>SSHVETRAHAEERLLKKLFSGYNKWSRPVANISDVVLVRFGLSIAQLIDVDEKNQMMTTNVWVKQEWHDYKLRWDPADYENVTSIRIPSELIWRPDIVLYNNADGDFAVTHLTKAHLFHDGRVQWTPPAIYKSSCSIDVTFFPFDQQNCTMKFGSWTYDKAKIDLVNMHSRVDQLDFWESGEWVIVDAVGTYNTRKYECCAEIYPDITYAFVIRRLPLFYTINLIIPCLLISCLTVLVFYLPSECGEKITLCISVLLSLTVFLLLITEIIPSTSLVIPLIGEYLLFTMIFVTLSIVITVFVLNVHHRSPRTHTMPTWVRRVFLDIVPRLLLMKRPSVVDTDFERSVKEDWKYVAMVIDRIFLWMFIIVCLLGTVGLFLPPWLAGMI[2x];>[3x]TDTEERLVEHLLDPSRYNKLIRPATNGSELVTVQLMVSLAQLISVHEREQIMTTNVWLTQEWEDYR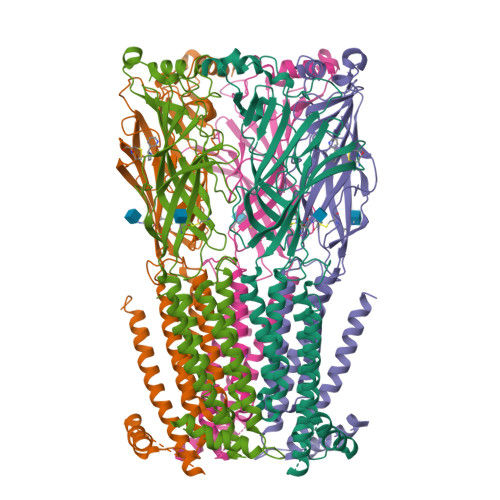LTWKPEEFDNMKKVRLPSKHIWLPDVVLYNNADGMYEVSFYSNAVVSYDGSIFWLPPAIYKSACKIEVKHFPFDQQNCTMKFRSWTYDRTEIDLVLKSEVASLDDFTPSGEWDIVALPGRRNENPDDSTYVDITYDFIIRRKPLFYTINLIIPCVLITSLAILVFYLPSDCGEKMTLCISVLLALTVFLLLISKIVPPTSLDVPLVGKYLMFTMVLVTFSIVTSVCVLNVHHRSPTTHTMAPWVKVVFLEKLPALLFMQQPRHHDDDQERSVSEDWKYVAMVIDRLFLWIFVFVCVFGTIGMFLQPLFQNYTTTTFLHSDHSAPSSKSAWSHPQFEK> MSLTLFHNPASPYVRKVMVLLHETGQ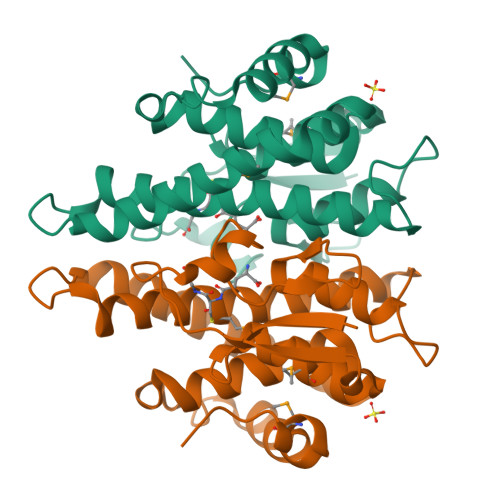LNRVALQASQLSPVAPDAALNQDNPLGKIPALRLDNGQVLYDSRVILDYLDQQHVGNPLIPRDGSARWRRLTLAALADGIMDASVLVRYELALRAPEKHWEQWLDGQRDKIRRALAVLEAEAIAELASHFDIAAISVACALGYLDFRHPDLEWRQDHPQLAAWYFEISQRPSMLATRPPVEGHHHHHH> GPVEDAVTAAIGRVADTVGTGPTNSEAIPALTAAETGHTSQVVPGDTMQTRHVKNYHSRSESTVENFLCRSACVYFTEYKNSGSKRYAEWVVTTRQAAQLRRKLEFFTYIRFDLELTFVITSTQQPSTTQNQDAQILTHQIMYVPPGGPVPDKVDSYVWQTSTNPSVFWTEGNAPPRMSIPFLSIGNAYSNFYDGWSDFSRDGVYGINTLNSMGTLYARHVNTGGTGPIKSTIRIYFKPKHVKAWIPRPPRLCQYEKAKNVNFQPSGVTTTRQSITAMTNT;> SPTVEECGYSDRVRSITLGNSTITTQECANVVVGYGVWPDYLKDNEATAEDQPTQPDVATCRFYTLDSVQWQKTSPGWWWKLPDALSNLGLFGQNMQYHYLGRTGYT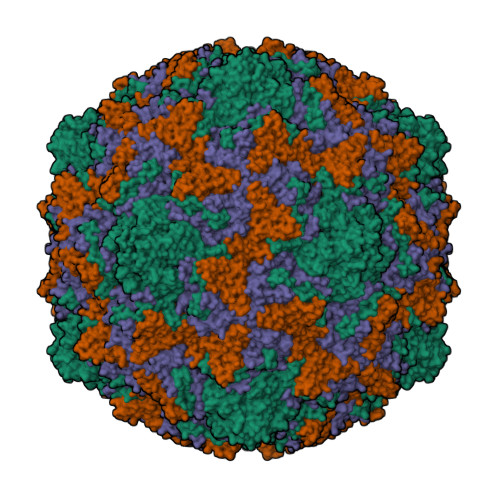IHVQCNASKFHQGCLLVVCVPEAEMGCATLDNTPSSAELLGGDAAKEFAGEPIASGSNKLVQRVVYNAGMGIGVGNLTIFPHQWINLRTNNSATIVMPYTNSVPMDNMFRHNNVTLMVIPFVPLDYCPGSTTYVPITVTIAPMNAEYNGLRLAGHQ;> GLPTMNTPGSCQFLTSDDFQSPSAMPQYDVTPEMRIPGEVKNLMEIAEVDSVVPVQNVGEKVNSMEAYQIPVRSNEGSGTQVFGFPLQPGYSSVFSRTLLGEILNYYTHWSGSIKLTFMFCGSAMATGKFLLAYSPLGAGAPTKRVDAMLGTHVVWDVGLQSSCVLCIPWISQTHYRYVASDECTAGGFITCWYQTNIVVPADAQSSCYIMCFVSACNDFSVRLLKDTPFISQENFFQ;> GAQVSTQKTGAHETGLNASGNSIIHYTNINYYKDAASNSATRQDFAQDPGKFTEPVKDIMIKSLPALN> 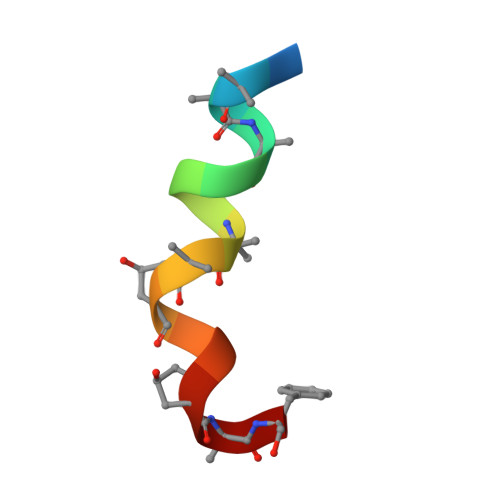XVAAAVGLAAPQVPAF The kink-turn (k-turn) is a widespread helical junction in RNA. The standard k-turn comprises a duplex RNA containing a three-nucleotide bulge followed by tandem G:A and A:G base pairs. The G:A base pairs adopt trans sugar-Hoogsteen conformation, also known as sheared base pairs, and the overall structure is tightly kinked, with an included angle between the axes of the flanking helices of 50°. In the absence of metal ions or binding proteins, the RNA adopts a conformation that is not tightly kinked, but rather bent in the manner of a simple three-nucleotide bulge. Many (but not all, see below) k-turns adopt the k-turn conformation on addition of divalent metal ions, but some will not.

The Actinomyces-1 sequence has −1b:−1n = C:G and 3b:3n = C:C, and was therefore predicted to undergo folding into the k-turn conformation on addition of Mg2+ ions. By contrast, Actinomyces-1 has 3b:3n = C:C which is predicted to confer the N1 conformation according to our conformational rules. The Actinomyces-1 k-turn sequence was inserted in place of the natural k-turn in the SAM-I riboswitch. We have previously found that this is a versatile vehicle for crystallizing many different k-turns, and accommodates k-turns in both the N3 and N1 conformation. The RNA adopts a standard k-turn geometry, with tandem trans-sugar-Hoogsteen G:A base pairs, and with both the cross-strand hydrogen bonds. However, in this case the hydrogen bond from G-1n O2′ is accepted by A2b N1. This requires the A2b nucleobase to rotate in plane so that the A2bN6 – G2nN3 distance is lengthened to 5.3 Å. The C:C base pair in the 3b:3n position is connected by a single hydrogen bond between C3bN4 and C3nO2. X-ray crystallography of the RAGATH-18 and Actinomyces-1 k-turns confirm that both form standard k-turn structures, with N3 and N1 conformations respectively.

> GGCUUAUCAAGAGAGGGCGAGGGACUGGCCCGACGACCCCCGGCAACCAGAAAUGGUGCCAAUUCCUGCAGCGGAAACGUUGAAAGAUGAGCCG> GPGHMTTLTRQDLNFGQVVADVLCEFLEVAVHLILYVREVYPVGIFQKRKKYNVPVQMSCHPELNQYIQDTLHCVKPLLEKNDVEKVVVVILDKEHRPVEKFVFEITQPPLLSISSDSLLSHVEQLLAAFILKISVCDAVLDHNPPGCTFTVLVHTREAATRNMEKIQVIKDFPWILADEQDVHMHDPRLIPLKTMTSDILKMQLYVEERAHKGS;> MWFPYDGSKLPLRPKRSPPVISEEAAEDVKQYLTI

The translesion synthesis (TLS) DNA polymerases Rev1 and Polζ function together in DNA lesion bypass during DNA replication, acting as nucleotide inserter and extender polymerases, respectively. It belongs to the B family of polymerases and is composed of subunits Rev3, Rev7, Pol31, and Pol32 (24, 25). The Polζ subunit Rev7 is a hub protein that directly binds Rev1 and is a component of several other protein complexes such as the shieldin DNA double-strand break repair complex. Rev7 is a member of the HORMA (Hop1, Rev7, and Mad2 proteins) domain protein family.

The structure of human Polζ is still unavailable, but we examined the crystal structures of human Rev7 in complex with fragments of shieldin-3 (SHLD3), including that with a SHLD3 peptide (41–74 aa), which we determined to a resolution of 2.0 Å to compare the binding modes of yeast and human Rev7. SHLD3 and Rev7 are two of the four components of the protein complex shieldin that plays a key regulatory role in DNA double-strand break repair by blocking DNA end resection necessary for homologous recombination. Since the two yeast Rev7 molecules have different organizations in the Polζ complex, we compared each to our human Rev7-SHLD3 crystal structure, which was determined in a Rev7 monomeric state using the R124A mutation. In the crystal structure of Rev7(R124A)-SHLD3, Rev7 binds the SHLD3 peptide at two sites. In one site, SHLD3 N-terminal loop residues P50 and L51 interact mainly via hydrophobic interactions with Rev7 residues A174, M160, and L173 in the safety-belt region of Rev7. In another hydrophobic interface, residues I60 and A65 in the C-terminal α-helix (αC-helix) of SHLD3 interact with Rev7 Y37 and P38. In human just like in yeast, Rev7 forms a homodimer, but the orientations of the two Rev7 protomers differ radically in the two systems. In yeast Rev7, the safety belt presents a short helix-turn-helix motif, but the one in human Rev7 is a short helix connected to a loop. The small backbone RMSDs with respect to Rev7A-Rev3RBM1 (RMSD 1.20 Å) and Rev7B-Rev3RBM2 (RMSD 1.08 Å) indicate that the yeast and human Rev7 folds are very similar. Although the yeast and human Rev7 proteins display virtually identical folds, their dimeric conformations and how they bind target proteins differ markedly.> VPQKPKVSLNPPWNRIFKGENVTLTCNGNNFFEVSSTKWFHNGSLSEETNSSLNIVNAKFEDSGEYKCQHQQVNESEPVYLEVFSDWLLLQASAEVVMEGQPLFLRCHGWRNWDVYKVIYYKDGEALKYWYENHNISITNATVEDSGTYYCTGKVWQLDYESEPLNITVI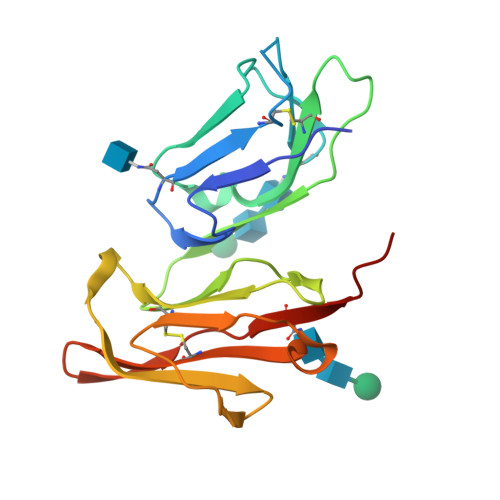KAPREK THYMIDINE-3'-PHOSPHATE | C10 H15 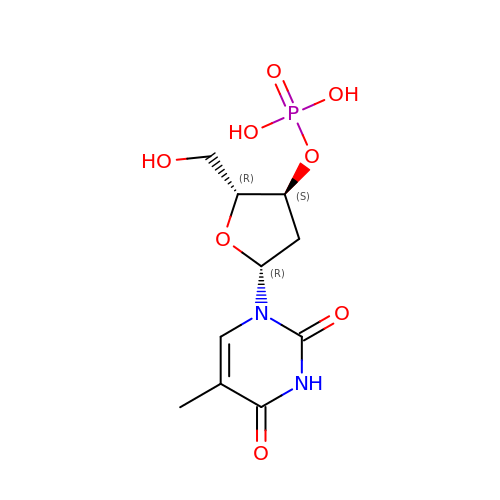N2 O8 P | XXYIANZGUOSQHY-XLPZGREQSA-N>AAQSVDIHKDQIIFSEGDAGDCAYIIEKGRVLIYLTKDKEEIPLTILGEGEIFGEMALIDNQNRSA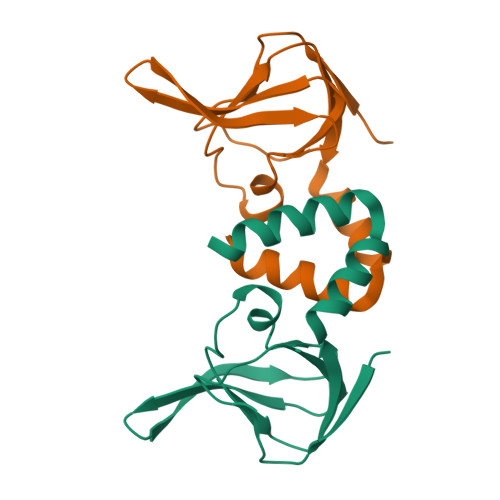SVRALEDVRLAIVTKQQVLERVSTADKVVQLLMRVLLKRLRR[2x]> RSVYELDCIPLWGVVSIQGNRSEMEDAFAVSPHFLKLPIKMLMGDHAGMSPSLTHLTGHFFGVYDGHGGHKVADYCRDRLHFALAEEIERIKDELCKRNTGEGRQVQWDKVFTSCFLTVDGEIEGKIGRAVVGSSDKVLEAVASETVGSTAVVALVCSSHIVVSNCGDSRAVLFRGKEAMPLSVDHKPDREDEYARIENAGGKVIQWQGARVFGVLAMSRSIGDRYLKPYVIPEPEVTFMPRSREDECLILASDGLWDVMNNQEVCEIARRRILMWHKKNGAPPLAERGK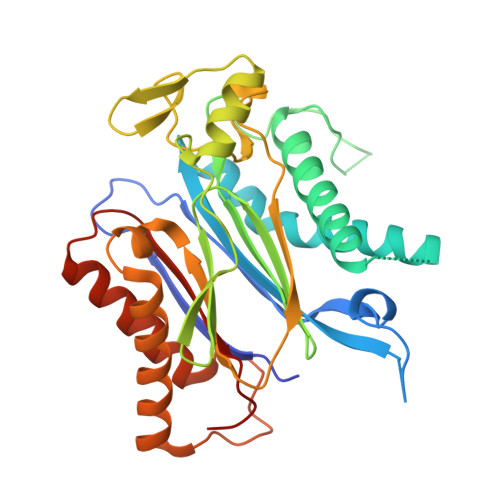GIDPACQAAADYLSMLALQKGSKDNISIIVIDLKAQRKFKTRT> MEKKITGYTTVDISQWHRKEHFEAFQSVAQCTYNQTVQLDITAF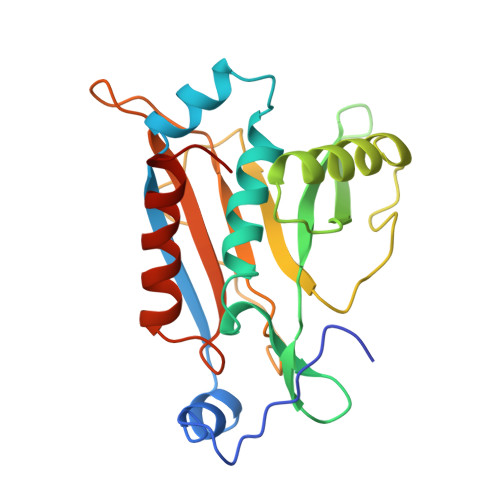LKTVKKNKHKFYPAFIHILARLMNAHPEFRMAMKDGELVIWDSVHPCYTVFHEQTETFSSLWSEYHDDFRQFLHIYSQDVACYGENLAYFPKGFIENMFFVSANPWVSFTSFDLNVANMDNFFAPVFTMGKYYTQGDKVLMPLAIQVHHAVCDGFHVGRMLNELQQYCDEWQGGA In general, transaminases catalyse the transfer of an amino group from an amino donor to a carbonyl acceptor with pyridoxal 5′-phosphate (PLP) as cofactor. Herein, we report the discovery of a new class of fold IV-transaminases, which was discovered during our quest for novel (R)-selective transaminases using an enrichment-based approach. In contrast to exclusive amino acid transaminases such as D-ATAs and BCATs, CpuTA1 and MgiTA1 are in addition able to convert amines to ketones, which would categorise them in the subclass of amine transaminases. Considering this and based on sequence and structural analysis, which revealed significant differences especially also in the active site, we propose that CpuTA1 and MgiTA1, might form a new subgroup in the fold IV family of PLP-dependent enzymes.

The crystal structure of CpuTA1 was determined by X-ray crystallography at a resolution of 2.4 Å. The final model contains 587 amino-acid residues (chain A and B), two pyridoxal-5′-phosphate (PLP), one 3-amino benzoic acid (3-ABA) and 327 water molecules. The asymmetric unit contains two polypeptide chains, which form a stable dimer with a contact surface of 5580 Å2 (PDBePISA29). CpuTA1 exhibits the typical aminotransferase type IV fold (InterPro: IPR001544, Pfam: Pf01063). The electron density for the PLP cofactor is well defined and the covalent imino bond to the active site Lys174 residue is clearly visible. The phosphate group is interacting through a network of hydrogen bonds to the side chains of Arg75, Thr234, Thr235 and Ser271, the backbone amides of Thr234, Thr235 and Ser271, and two water molecules. The two active sites are located at the interface of the two polypeptide chains with the main portion located in one chain, and vice versa. The active site is surrounded by the residues R51*, F56, T58, F115, K117, E125, E140, F142, Y178, S270, S271, and V272 (*indicates that the residues belongs to the other chain). These amino acids are building two binding pockets, whereby the small binding pocket is lined by T58, S270, S271 and V272 and the large binding pocket by R51*, F56, K115, E125*, E140, F142 and Y178. Overall, the structure of CpuTA1 confirms that except for the PLP binding amino acids hardly any of the active site amino acids is conserved compared to the characterised fold IV subgroups. Interestingly, a flexible loop (e.g. aa K125-I135 in AT-ωTA), which is present in (R)-ATAs13151735 as part of the active site (the loop of chain B as part of the active site of chain A and vice versa containing an arginine residue, which is discussed to play a role in dual substrate recognition of (R)-ATAs131535) is significantly shorter in CpuTA1 (aa E125-G128) and does not contain any positively charged amino acid.

>[2x]MTRATLLTVTAPTRPASADEHGADRAAGDAGFVLADFGAPQVRITDLGITRGDGVFETIAVIDGHPQALELHLGRLAHSAALLDLPEPDAAVWREAVLAGVADYRSRNGDGGELFAKLILTRGIEGEGRPSGWVFVDEGEDFSQQRLGIRVVTLDRGYRHDVAETSPWLLAGAKSLSYATNRAAGREAARRGADDVIFVSSDGYALEGPTSNVIVLADGVVRTPQTDQGILAGTTQAAVFDFFEERGYPTEYRRISADELRDAEALWLVSSVRQAAPITALDDREYPVDAALTADLNAYLLARTDLEHHHHHH>[2x]VPVVGIVAALLPEMGIGFQGNLPWRLAKEMKYFREVTTLTNDNSKQNVVIMGRKT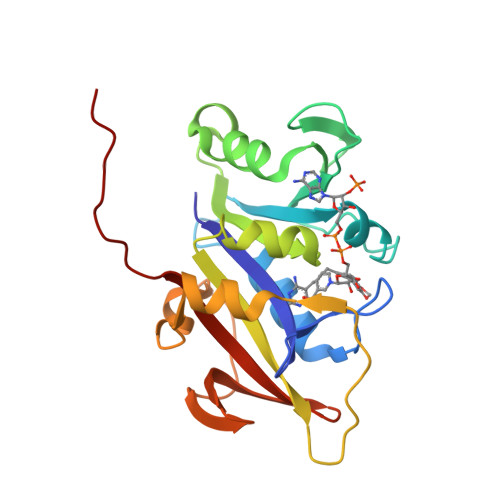WESIPQKFRPLPKRINVVVSRSFDGELRKVEDGIYHSNSLRNCLTALQSSLANENKIERIYIIGGGEIYRQSMDLADHWLITKIMPLPETTIPQMDTFLQKQELEQRFYDNSDKLVDFLPSSIQLEGRLTSQEWNGELVKGLPVQEKGYQFYFTLYTKKLEHHHHHHHH>[2x]CG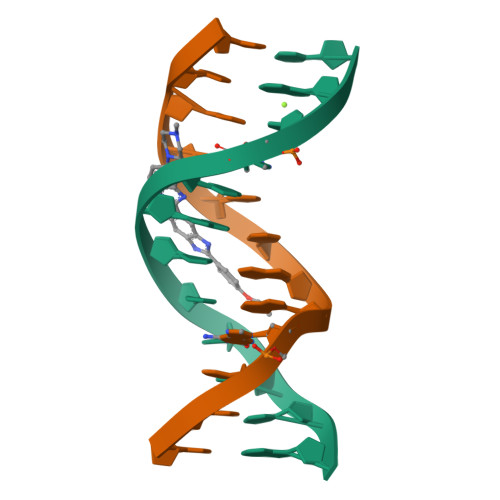CGAATTTGCG>[6x]GMFEKQFNHRTLETSLGPVEIEGPVTSQILATYKLDPGLTAFRQPAEQH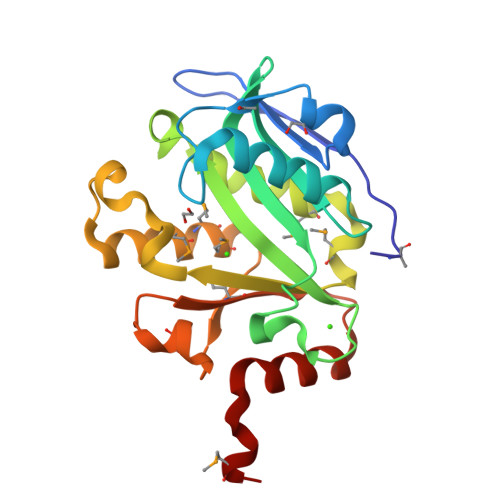EALVEIAALEEGRIIIARQGNDIIGYVTFLYPDPYETWSEGNNPYILELGAIEVAARFRGQQIGKKLLEVSMLDPAMEHYLILTTEYYWHWDLKGSGLSVWDYRKIMEKMMNHGGLVFFPTDDPEIASHPANCLMARIGKHVAPEVVAHFDALRLRRRFMYD>[6x]MERLDIFGVPIDRVTMIQAVDILNNFLQENRLHIVATPNAEIVMMAQKDKEYMEILNNTDLNVPDGSGIVFASKVFKKPLPERVAGFDLM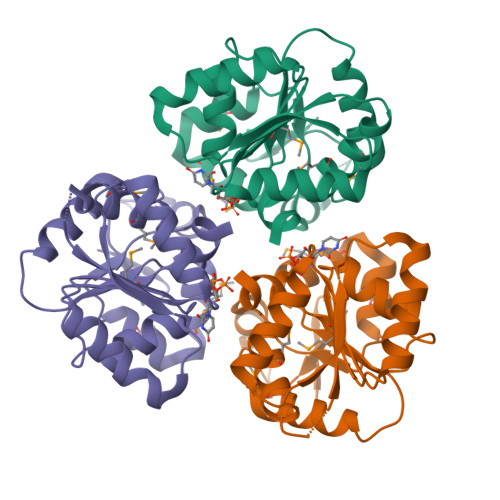LEFIKGISSKGVKIYLLGAACQVAEQARANLEKLYPGVKIVGTHHGYFTEEEENKIIEEINNKGAEVLFVALGAPKQEKWIYKNKDKLKVKIAMGVGGSFDVIAG> GPGSCPTHADSLNNLANIKREQGNIEEAVRLYRKALEVFPEFAAAHSNLASV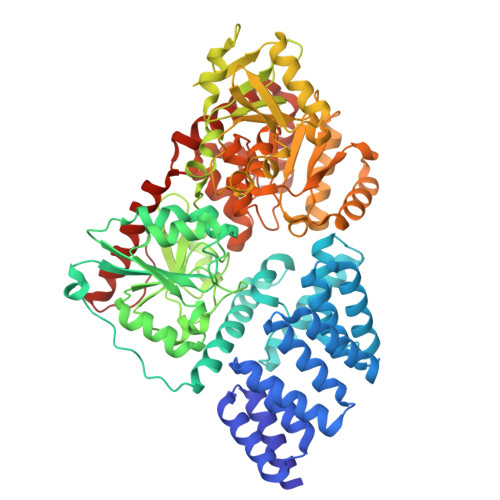LQQQGKLQEALMHYKEAIRISPTFADAYSNMGNTLKEMQDVQGALQCYTRAIQINPAFADAHSNLASIHKDSGNIPEAIASYRTALKLKPDFPDAYCNLAHCLQIVCDWTDYDERMKKLVSIVADQLEKNRLPSVHPHHSMLYPLSHGFRKAIAERHGNLCLDKINVLHKPPYEHPKDLKLSDGRLRVGYVSSDFGKHPTSHLMQSIPGMHNPDKFEVFCYALSPDDGTNFRVKVMAEANHFIDLSQIPCNGKAADRIHQDGIHILVNMNGYTKGARNELFALRPAPIQAMWLGYPGTSGALFMDYIITDQETSPAEVAEQYSEKLAYMPHTFFIGDHANMFPHLKKKAVIDFKSNGHIYDNRIVLNGIDLKAFLDSLPDVKIVKMKCPDGGDNADSSNTALNMPVIPMNTIAEAVIEMINRGQIQITINGFSISNGLATTQINNKAATGEEVPRTIIVTTRSQYGLPEDAIVYCNFNQLYKIDPSTLQMWANILKRVPNSVLWLLRFPAVGEPNIQQYAQNMGLPQNRIIFSPVAPKEEHVRRGQLADVCLDTPLCNGHTTGMDVLWAGTPMVTMPGETLASRVAASQLTCLGCLELIAKNRQEYEDIAVKLGTDLEYLKKVRGKVWKQRISSPLFNTKQYTMELERLYLQMWEHYAAGNKPDHMIKPVE>[3x]MGQGPELHLASQFVNEACRALVFGGCVEKSSVSRNPEVPFESSAYRISASARGKELRLILSPLPGAQPQQEPLALVFRFGMSGSFQLVPREELPRHAHLRFYTAPPGPRLALCFVDIRRFGRWD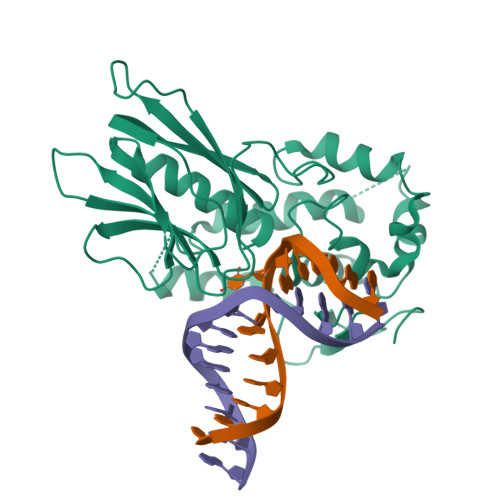LGGKWQPGRGPCVLQEYQQFRENVLRNLADKAFDRPICEALLDQRFFNGIGNYLRAEILYRLKIPPFEKARSVLEALQQHRPSPELTLSQKIRTKLQNPDLLELCHSVPKEVVQLGGRGYGSESGEEDFAAFRAWLRCYGMPGMSSLQDRHGRTIWFQGDPGPLAPKGRKS> MTRVRQALVALCALSLTFVTVSASASADPRETVSADAAETGSATESRPGILGTWYNQLGSVMVVTRAANGGFVGTYESAVGNAEKRYVMTGRYDSAPADGTGTAVGWTVAYRNAHRNAHSVATWSGQYVGGSQERIVTQWLLSYGTTPADQWKSTFLGHDEFTRVKPSAADVEKARQLGVTSANPPASDGE

The members of the avidin protein family are well known for their high affinity towards d-biotin and their structural stability. In the present study, two avidin-like biotin-binding proteins (named streptavidin C1 and C2) from Streptomyces cinnamonensis were newly identified while exploring antifungal proteins against Fusarium oxysporum f. sp. cucumerinum. Streptavidin C1 reveals a low correlation (a sequence identity of approximately 64%) with all known streptavidins, whereas streptavidin C2 shares a sequence identity of approximately 94% with other streptavidins. Here, the crystal structures of streptavidin C1 in the mature form and in complex with biotin at 2.1 and 2.5 Å resolution, respectively, were assessed.

Similar to other streptavidin family members, four sets of interactions are present in the biotin-binding sites. Firstly, a hydrogen-bonding network with biotin is formed by Asn56, Ser60, Tyr76, Ser78 and Asp160. The second set of interactions comprises hydrophobic interactions between biotin and strictly conserved residues (Leu58 in Loop1–2, Val80 in Loop3–4, Tyr111 in Loop5–6, Trp140 in β7 and Leu142 in β7). Tyr111 in Loop5–6 is a specific novel residue that interacts with d-biotin, and in most proteins of the (strept)avidin family this position is occupied by a tryptophan residue, except for tamavidin, which has a phenylalanine at this position. We did not find electron density for the ECP and C-Lid regions when biotin was bound to the protein, which indicates that these regions are flexible but do not affect the binding ability of biotin. d of biotin binding to recombinant streptavidin C1 was about 3.06 ± 0.498 pM. r value of streptavidin C1 is lower than that of streptavidin C2 and the reported values for streptavidin, bradavidin and tamavidin. Moreover, streptavidins C1 and C2 with d-biotin exhibited thermal stability even at 100°C and mostly remained in the tetrameric form [Supplementary Figs. S3(c) and S3(d)].>ESEHTEVSLALFNYDDINVKVDFILLEKNMTINELKMYVENELFKFPDDIVKHVNIKVNGSLVGHGELVSIEDGYGI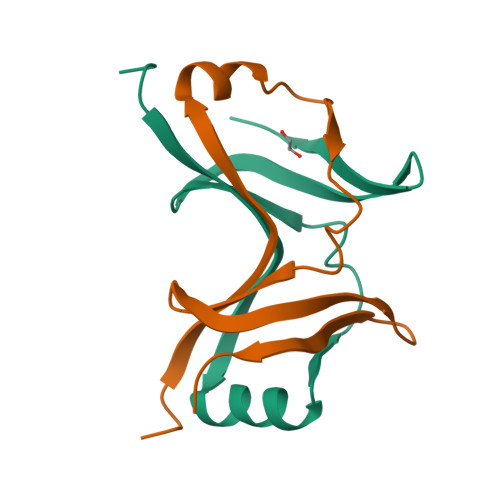EISSWMVKE[4x]palonosetron | C19 H24 N2 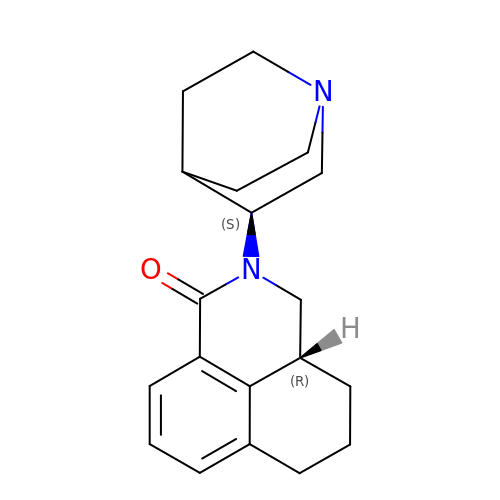O | CPZBLNMUGSZIPR-DOTOQJQBSA-N> MATSSMSKGCFVFKPNSKKRKISLPIEDYFNKGKNEPEDSKLRFETYQLIWQQMKSENERLQEELNKNLFDNLIEFLQKSHSGFQKNSRDLGGQIKLREIPTAALVLGVNVTDHDLTFGSLTEALQNNVTPYVVSLQAKDCPDMKHFLQKLISQLMDCCVDIKSKEEESVHVTQRKTHYSMDSLSSWYMTVTQKTDPKMLSKKRTTSSQWQSPPVVVILKDMESFATKVLQDFIIISSQHLHEFPLILIFGIATSPIIIHRLLPHAVSSLLCIELFQSLSCKEHLTTVLDKLLLTTQFPFKINEKVLQVLTNIFLYHDFSVQNFIKGLQLSLLEHFYSQPLSVLCCNLPEAKRRINFLSNNQCENIRRLPSFRRYVEKQASEKQVALLTNERYLKEETQLLLENLHVYHMNYFLVLRCLHKFTSSLPKYPLGRQIRELYCTCLEKNIWDSEEYASV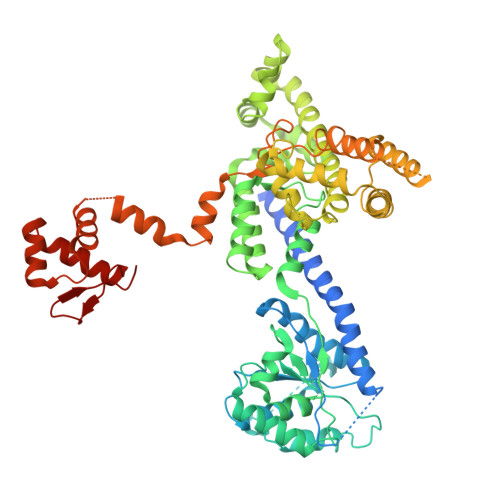LQLLRMLAKDELMTILEKCFKVFKSYCENHLGSTAKRIEEFLAQFQSLDAETKEEEDASGSQPKGLQKTDLYHLQKSLLEMKELRRSKKQTKFEVLRENVVNFIDCLVREYLLPPETQPLHEVVYFSAAHALREHLNAAPRIALHTALNNPYYYLKNEALKSEEGCIPNIAPDICIAYKLHLECSRLINLVDWSEAFATVVTAAEKMDANSATSEEMNEIIHARFIRAVSELELLGFIKPTKQKTDHVARLTWGGC>MAKKTSSKGKLPPGPRPLPLLGNLLQMDRRGLLKSFLRFREKYGDVFTVHLGPRPVVMLCGVEAIREALVDKAEAFSGRGKIAMVDPFFRGYGVIFANGNRWKVLRRFSVTTMRDFGMGKRSVEERIQEEAQCLIEELRKSKGALMDPTFLFQSITANIICSIVFGKRFHYQDQEFLKMLNLFYQTFSLISSVFGQLFELFSGFLKHFPGAHRQVYKNLQEINAYIGHSVEKHRETLDPSAPRDLIDTYLLHMEKEKSNAHSEFSHQNLNLNTLSLFFAGTETTSTTLRYGFLLMLKYPHVAERVYREIEQVIGPHRPPELHDRAKMPYTEAVIYEIQRFSDLLPMGVPHIVTQHTSFRG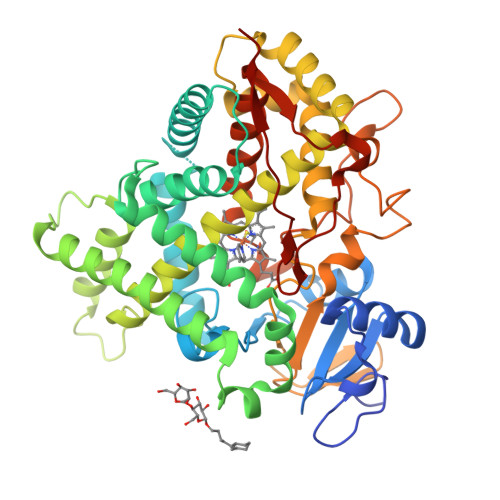YIIPKDTEVFLILSTALHDPHYFEKPDAFNPDHFLDANGALKKTEAFIPFSLGKRICLGEGIARAELFLFFTTILQNFSMASPVAPEDIDLTPQECGVGKIPPTYQIRFLPRHHHH[6x]> AFVVTDNCIKCKYTDCVEVCPVDCFYEGPNFLVIHPDECIDCALCEPECPAQAIFSEDEVPEDMQEFIQLNAELAEVWPNITEKK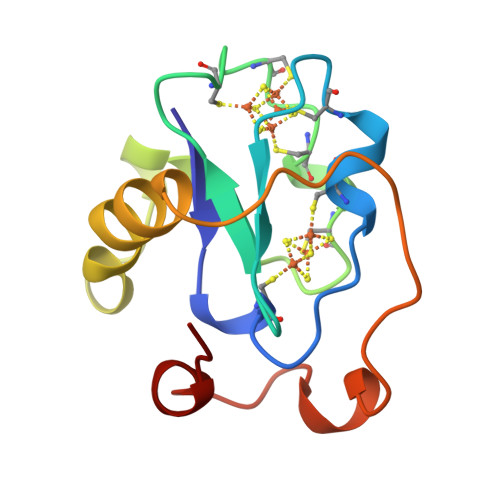DPLPDAEDWDGVKGKLQHLER> MAIAFEHVTYTYQAGTPMAHTALTDVSLTVPDRGYLAIIGHTGSGKSTLIQQLNALLKPTSGTIKIDEFTITPETTNAALKPLRQHVGMVFQFPENQLFEETVRQDIAFGPKNFGMADADALALADEMLTTVGLDQSYAERSPFELSGGQMRRVAIAGVLAMQPKVLVLDEPTAGLDPQGRQEMMRLFARLHQEQGLTIVLVTHQMEDVAQYAEQVAVMHEGRLMKFGTPADVFSNREWLQDHQLDVPQAAQFARRLRDRGLTFPKQPLTADQLADYLAQQWAQRGADHV;> MTENIISVDHLTYQYDENQAPALTDVSFTVHAGEWLAIVGHNGSGKSTLAKSLDGLLPFTQGSVTVGGITLTPETVWQVREQIGMIFQNPDNQFVGATVEDDVAFGLENRQISRDEMVPRVQAALAQVGMTSFAQREPSSLSGGQKQRVALAGIVAIAPKILILDEATSMLDPQGRIEMLAIVRQLRQQQNLTVISITHDIDEAASADRVLVIDDGRLVDEAVPSQIFERGTQLVEMGLDLPFTEKLKAALRQRGITPPTTYQTAAEMEEWLWQSLSNT;> MAKTQLPK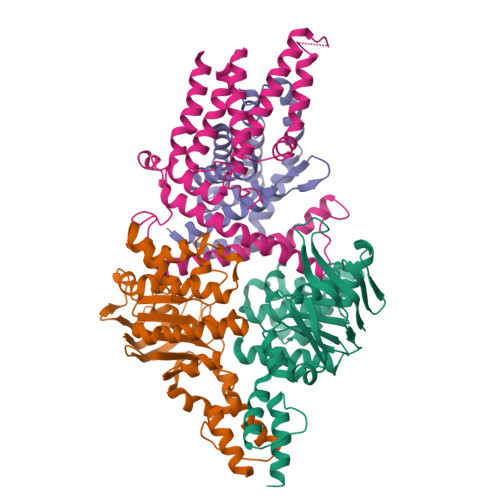LDTLSMVTMGVLMALQLVISRFSVGNNFIKVSFTFLIVALIAKWFGPWWGMLTAAVVDVIGTLMTGGPFFIGFTVSAVLGSLIYAVFLYRQPVSWWRVIGASVLIALLVNTLLNTLWVTIMYQTPFWSLLPVRALKELIVTPVQIVLVYLLLKSQVIQMIQARLNK;> MGSSHHHHHHSQDPMSNFIFGRYLPLDSVVHRLDPRAKLMLSFCYIIVVFLANNIWSYAILIAFTVGAILSSKISLGFFLKGIRPLLWLIVFTVVLQLLFSPAGGHTYFHWAFINVTQDGLINAGYIFVRFLLIIMMSTLLTLSTQPLDIATGLASLMKPLRWVKVPVDTLAMMLSIALRFVPTLMDEATKIMNAQRARGVDFGEGGLFKQAKSLIPLMVPLFMSAFNRAEDLSTAMEARGYQDSEHRSQYRILTWQRRDTVTWLLFLLGFVAILIFRHW>GAMADIGSMKTVGYAIVGTGYFGAELGRIMKEQEGARIVAVLDPENGQTIAEELDCDVETDLDTLYSREDVEAVIVATPNYLHKEPVIKAAEHGVNVFCEKPIALSYQDCDEMVRTCQEHGVIFMAGHVMNFFHGVRYAKKLINDGVIGKVLYCHSARNGWEEQQPTISWKKIREKSGGHLYHHIHELDCVQFLMGGMPEEVTMTGGNVAHQGEAFGDEDDMLFVNMQFSDNRYAVLEWGSAFHWPEHYVLIQGTKGAIKIDMCDCGGTLKVDGREEHFLVHESQ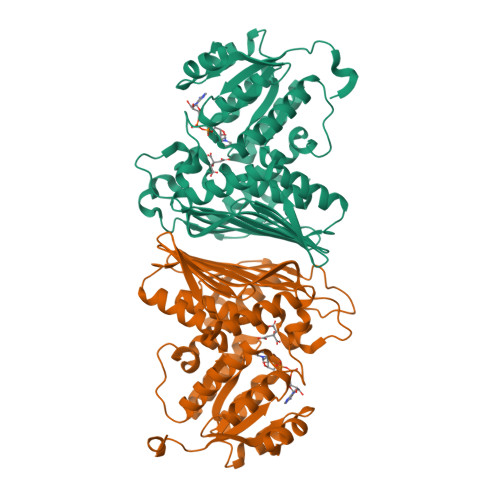EEDDDRTRIYHGTEMDGAIMYGKPGKKPPMWLHSIMKNEMKYLNGILHGKEVDDEFRPLLTGEAARAAIATADACTKSRFEDRKVKLSEIIGEGSTI[2x]> MPKRIVYNISSDFQLKSLLGEGAYGVVCSATHKPTGEIVAIKKIEPFDKPLFALRTLREIKILKHFKHENIITIFNIQRPDSFENFNEVYIIQELMQTDLHRVISTQMLSDDHIQYFIYQTLRAVKVLHGSNVIHRDLKPSNLLINSNCDLKVCDFGLARIIDESAADNSEPTGQQSGMVEFVATRWYRAPEVMLTSAKYSRAMDVWSCGCILAELFLRRPIFPGRDYRHQLLLIFGIIGTPHSDNDLRCIESPRAREYIKSLPMYPAAPLEKMFPRVNPKGIDLLQRMLVFDPAKRITAKEALEHPYLQTYHDPNDEPEGEPIPPSFFEFDHYKEALTTKDLKKLIWNEIFS;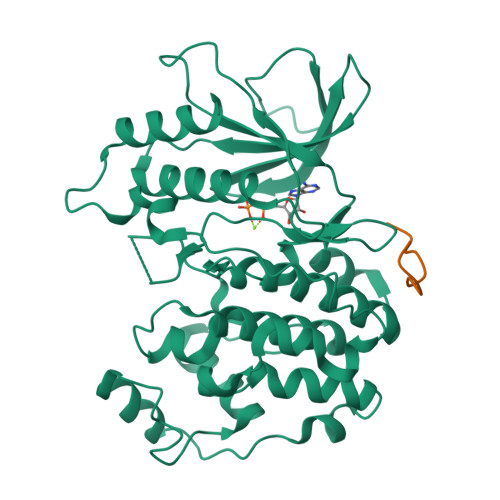> SKRGNIPKPLNLS>[14x]MGSSHHHHHHSSGRENLYFQGHM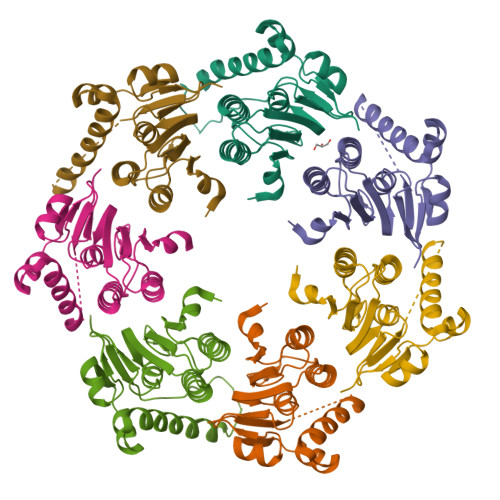SYNEHHKYNINIPSLLLSKRIIFLSSPIYPHISEQIISQLLYLEYESKRKPIHLYINSTGDIDNNKIINLNGITDVISIVDVINYISSDVYTYCLGKAYGIACILASSGKKGYRFSLKNSSFCLNQSYSIIPFNQATNIEIQNKEIMNTKKKVIEIISKNTEKDTNVISNVLERDKYFNADEAVDFKLIDHILEKE>SNILEMTKNYYDRSVSPVEYAYFDQSQNMRAINWNKIVDEKDLEVWNRVTQNFWLPENIPVSNDLPSWNELDDDWQQLITRTFTGLTLLDTVQSSIGDVAQIKNSLTEQEQVIYANFAFMVGVHARSYGTIFSTLCTSEQIEEAHEWVVDNEALQARPKALIPFYTADDPLKSKIAAALMPGFLLYGGFYLPFYLSARGKLPNTSDIIRLILRDKVIHNFYSGYKYQLKVAKLSPEKQAEMKQFVFDLLDKMIGLEKTYLHQLYDGFGLADEAIRFSLYNAGKFLQN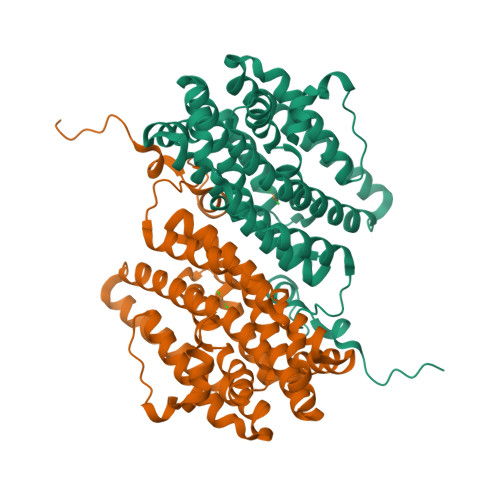LGYESPFTKEETRIAPEVFAQLSARADENHDFFSGSGSSYIIGTSEETLDEDWDF[2x]> MATAALKSFKPKQPHKANFWFMLGIEDAETGRTDAVHKGFEPKVYRNIVERVKLSQNEFQNVTLIPVSTIKRRLKNDERFNTQESDAIYRLAMLLKLATELFDDEERALEWMKENVYGLGGKRPLDMV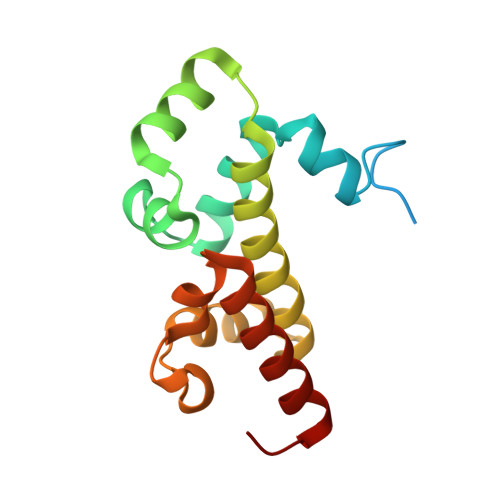STTVDFEIVKDLIGRLEHGVFS>[4x]QVVSQGWKYFKGNFYYFSLIPKTW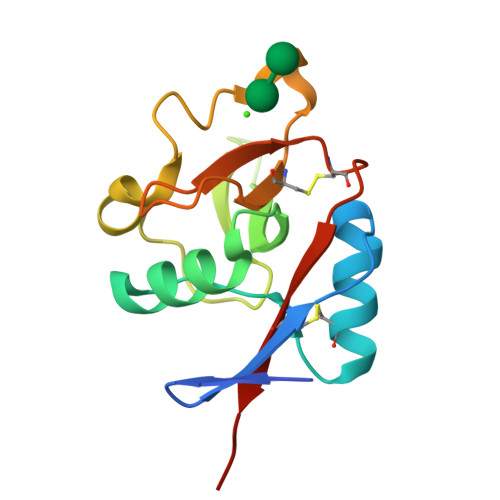YSAEQFCVSRNSHLTSVTSESEQEFLYKTAGGLIYWIGLTKAGMEGDWSWVDDTPFNKVQSARFWIPGEPNNAGNNEHCGNIKAPSLQAWNDAPCDKTFLFICKRPYVPSEP> MKHHHHHHMKQNSPLDEENLTQENQDRGTHVDRGLASANVDFAFSLYKQLVLKAPDKNVIFSPLSISTALAFLSLGAHNTTLTEILKGLKFNLTETSEAEIHQSFQHLLR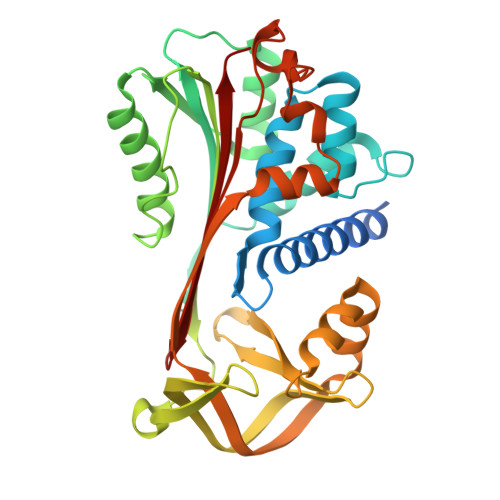TLNQSSDELQLSMGNAMFVKEQLSLLDRFTEDAKRLYGSEAFATDFQDSAAAKKLINDYVKNGTRGKITDLIKDLDSQTMMVLVNYIFFKAKFEMPFDPQDTHQSRFYLSKKKYVMVPMMSLHHLTIPYFRDEELSCTVVQLNYTGNASALFILPDQDKMEEVEAMLSQETLSRFFDSLEFREIGELYLPKFSISRDYNLNDILLQLGIEEAFTSKADLSGITGARNLAVSQVVHKAVLDVFEEGTERSAATALKGPRQ> SMKMMLDKKQIRAIFLFEFKMGRKAAETTRNMNNAFGPGTANERTVQWWFKKFRKGDESLEDEERSGRPSEVDNDQLRAIIEADPLTTTREVAEEM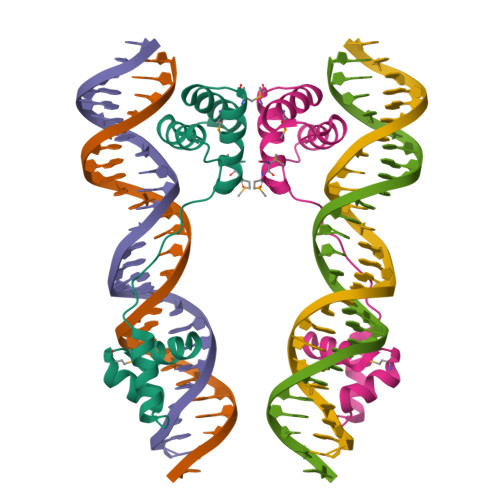NVNHSTVVRHLKQIGKV>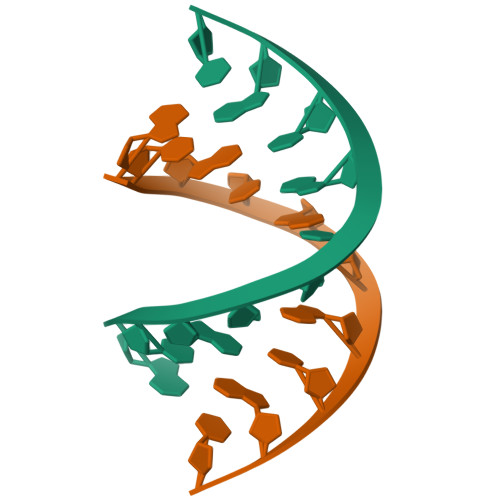 GCACGCGTGC> SVGADLGLWNRLEPALAYLAPEERAKVREAYRFAEEAHRGQLRRSGEPYITHPVAVAEILAGLQMDADTVAAGLLHDTLEDCGVAPEELERRFGPTVRRIVEGETKVSKLYKLANLEGEERRAEDLRQMFIAMAEDVRIIIVKLADRLHNLRTLEHMPPEKQKRIAQETLEIYAPLAHRLGMGQLKWELEDLSFRYLHPEAFASLSARIQATQEARERLIQKAIHLLQETLARDELLQSQLQGFEVTGRPKHLYSIWKKMEREGKTLEQIYDLLAVRVILDPKPAPTRESQALREKQVCYHVLGLVHALWQPIPGRVKDYIAVPKPNG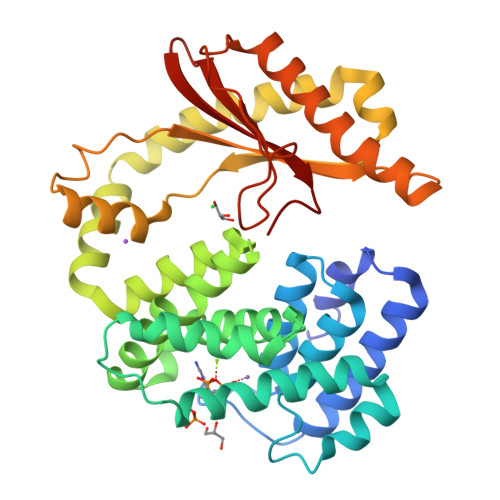YQSLHTTVIALEGLPLEVQIRTREMHR>GAMGEHNQKKEIKEEDFFPSTEEEKQADKAIKDIENLIGESGFPELIENVCSLKHEYTLIRSDFYDVITKIQNKKISLMKNSHNNRNKIRELVQLQNNLKIGDELDKIMGCIDTAEQEIRSAAFFFDEAKESLKEGIIKRLEKSKNRAASQLSKKALNRAEDALRCLENYSSKK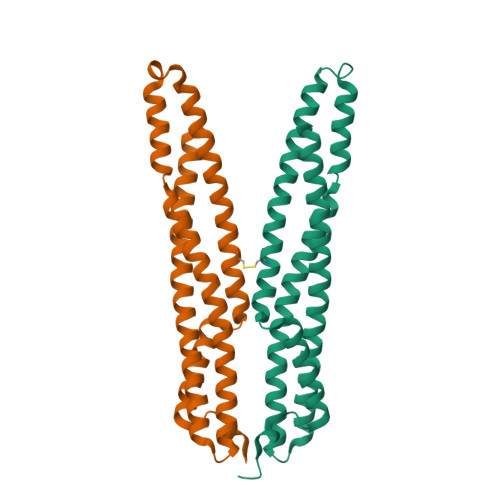GEAIGRRSFIKEVVEQAKNALSKS[2x]> MGSSHHHHHHSSGRENLYFQGHMEKTVIYLLEDGYVDFVVEKIRTKMEKLLEEKDKIFVVLAGGRTPLPVYEKLAEQKFPWNRIHFFLSDERYVPLDSDQSNFRNINEVLFSRAKIPSGNVHYVDTSLPIEKACEKYEREIRSATDQFDLAILGMGPDGHVASIFDLETGNKDNLVTFTDPSGDP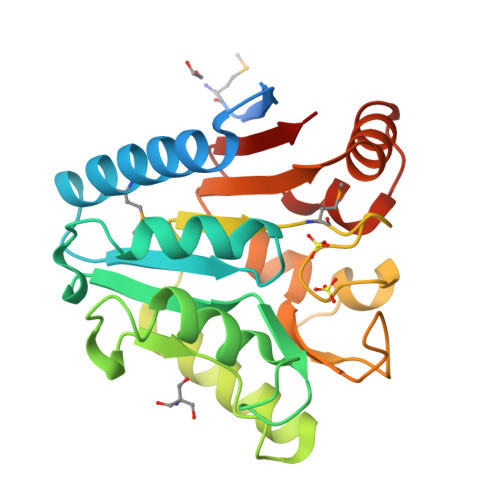KVPRVTLTFRALNTSLYVLFLIRGKEKINRLTEILKDTPLPAYFVRGKEKTVWFVGKGS> GPGSRAAQGRAFGNLGNTHYLLGNFRDAVIAHEQRLLIAKEFGDKAAERIAYSNLGNAYIFLGEFETASEYYKKTLLLARQLKDRAVEAQSCYSLGNTYTLLQDYEKAIDYHLKHLAIAQELKDRIGEGRACWSLGNAYTALGNHDQ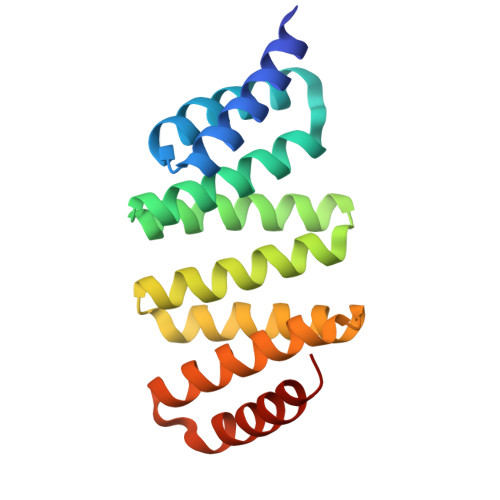AMHFAEKHLEISREVGD> GHMTGADTEAVVCVGTACYTAHSGKLSAAEAQNHCNQNGGNLATVKSKEEAQHVQRVLAQLLRREAALTARMSKFWIGLQREKGKCLDPSLPLKGFSWVGGGEDTPYSNWHKELRNSCISKRCVSLLLDLSQPLLPSRLPKWSEGPCGSPGSPGSNIEGFVCKFSFKGMCRPLALGGPGQVTYTTPFQTTSSSLEAVPFASAANVACGEGDKDETQSHYFLCKEKAPDVFDWGSSGP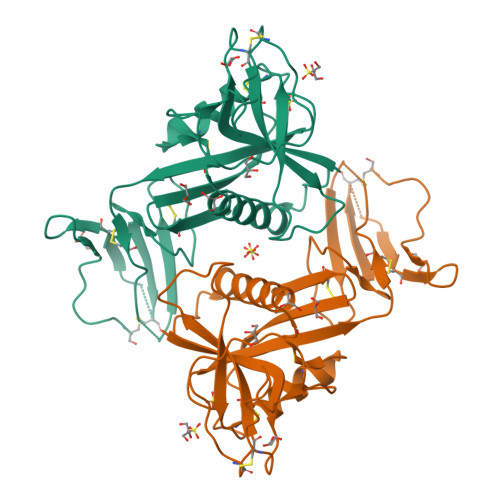LC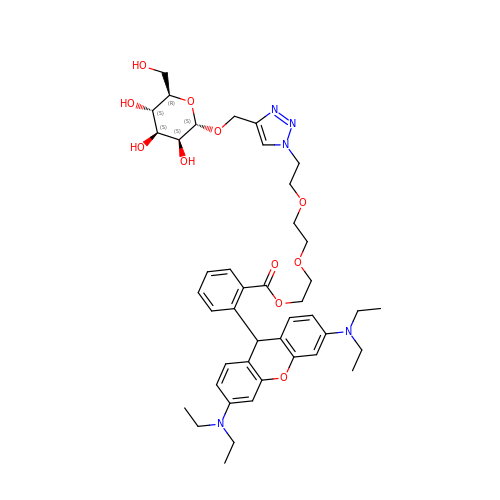2-[2-(2-{4-[(alpha-D-mannopyranosyloxy)methyl]-1H-1,2,3-triazol-1-yl}ethoxy)ethoxy]ethyl 2-[3,6-bis(diethylamino)-9H-xanthen-9-yl]benzoate | C43 H57 N5 O11 | LPSYXQPVOZLKRL-VWIMFXPFSA-N> GPLGSEQLKCCSGILKEMFAKKHAAYAWP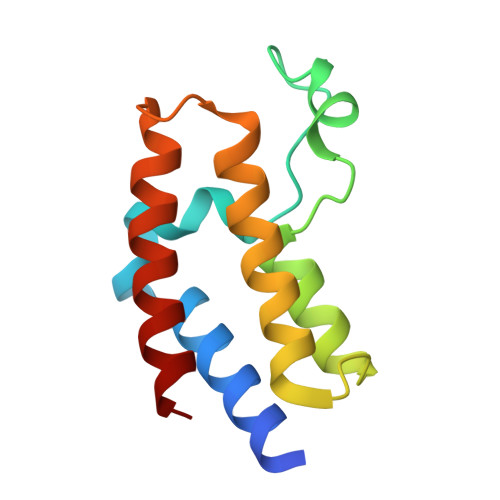FYKPVDVEALGLHDYCDIIKHPMDMSTIKSKLEAREYRDAQEFGADVRLMFSNCYKYNPPDHEVVAMARKLQDVFEMRFAKM> KPISPEQEELIHRLVYFQNEYEQPSDEDFRHITEITILTVQLIVEFAKRLPGFDKLLREDQIALLKACSSEVMMLRMARRYDVGSDSILATVDDLLRFCRQMYGMKVDNAEYALLTAIVIFSERPSLIEGWKVEKIQEIYLEALKVYVDNRRKPRSGTIFAKLLSVLTELRTLGNLNSEMCFSLKL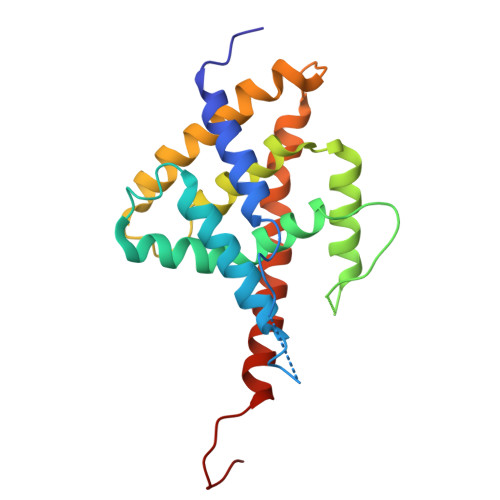KNKKLPPFLAE5-azanyl-[1,3]thiazolo[5,4-d]pyrimidine-2,7-dione | C5 H2 N4 O2 S | 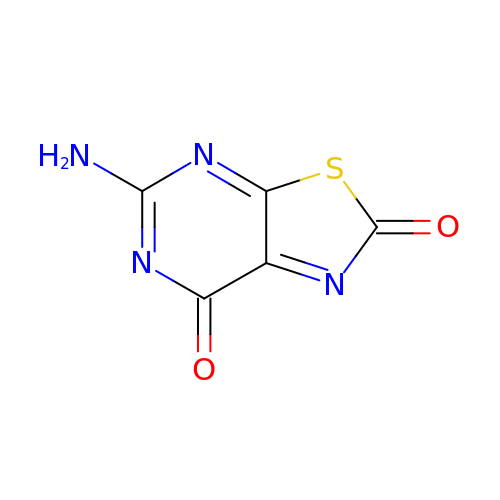AXABAVYDNQCEBU-UHFFFAOYSA-N[(2~{R},3~{S},4~{S})-3,4-bis(oxidanyl)oxolan-2-yl]methyl phosphono hydrogen phosphate | C5 H12 O10 P2 | 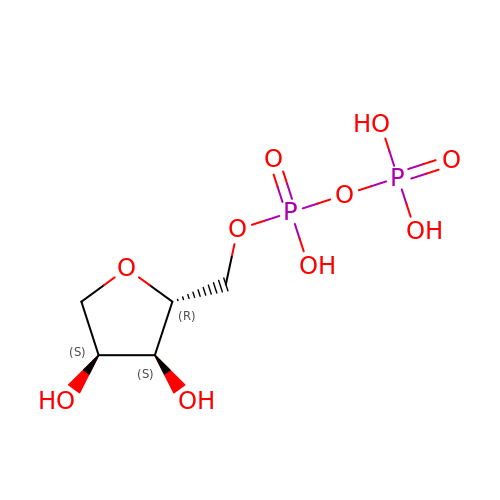HNPYBPXXPMVWIY-LMVFSUKVSA-N N~6~-methyl-N~6~-[4-(propan-2-yl)phenyl]pyrido[2,3-d]pyrimidine-2,4,6-triamine 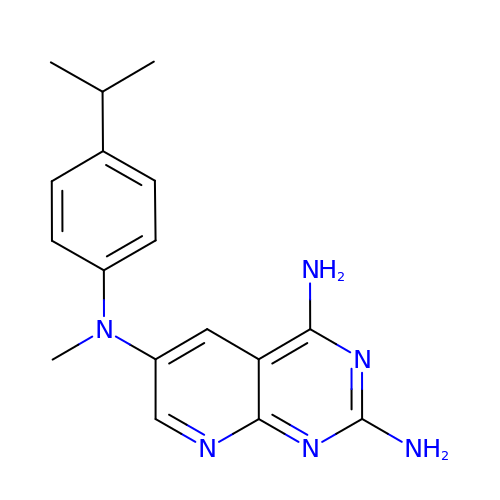| C17 H20 N6 | CRSDIJKYSOUKQH-UHFFFAOYSA-N>[4x]MADQEHIDAGLLSTNFDMIQALPLNVKQRVCALKNLQMKTIQIESDFYKRVHELEIEFEGKFKSTFDQRKAIVAGEVEPTKEQIDTPILEGLEGDQLAELYKAAEADPSAKGIKDF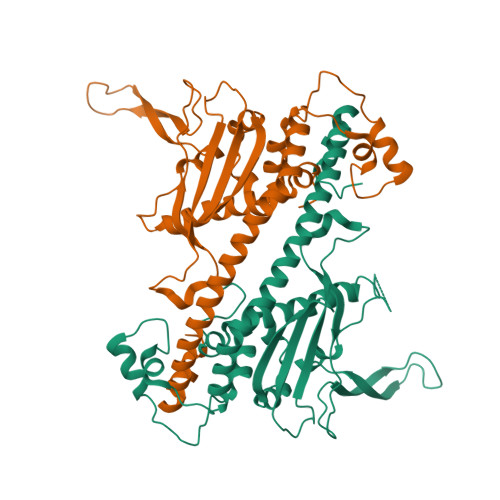WLTALRTHDLVAEAIEEHDVPILSYLTDVTTAASKDPAGFKIEFHFATNPYFKNQVLTKTYLLGFDPDAEAPLQFDGPHVIRAVGDTIEWEDGKNVTKKAVKKKQKKGANAGKFLTKTVKADSFFNFFEPPKSKDERNEDEDDEQAEEFLELDYEMGQAIRDTIIPRAVLFYTGELQSDDMFDFPGEDGDDVSDFSDDEA>[4x]SNAMYQHRDWQGALLDFPVNKVVCVGSNYAEHIKEMGSTASVEPVLFIKPE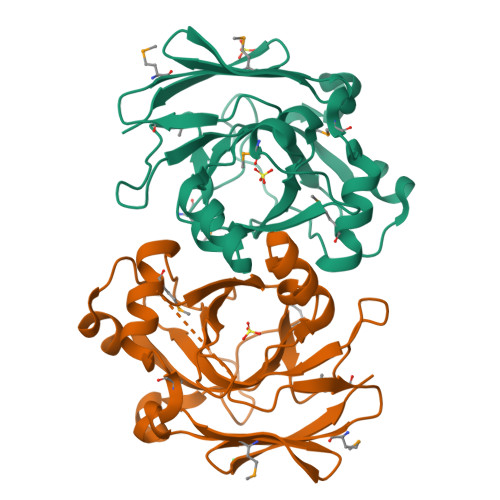TALCDIRQPVSIPKDFGSVHHEIELAVLIGTPLKQASEDRVARAIAGYGVALDLTLRELQAGFKKAGQPWEKAKAFDGSCPISGFIPVAEFGDAQQADLSLTINGEIRQQGNTRDMITPIIPLISYMSRFFTLRAGDIVLTGTPQGVGPMQSGDMLKIMLNGKTVNTRII>MSKVPSDIEIAQAAKMKPVMELARGLGIQEDEVELYGKYKAKISLDVYRRLKDKPDGKLILVTAITPTPAGEGKTTTSVGLTDALARLGKRVMVCLREPSLGPSFGIKGGAAGGGYAQVVPMEDINLHFTGDIHAVTYAHNLLAAMVDNHLQQGNVLNIDPRTITWRRVIDLNDRALRNIVIGLGGKANGVPRETGFDISVASEVMACLCLASDLMDLKERFSRIVVGYTYDGKPVTAGDLEAQGSMALLMKDAIKPNLVQTLENTPAFIHGGPFANIAHGCNSIIATKTALKLADYVVTEAGFGADLGAEKFYDVKCRYAGFKPDATVIVATVRALKMHGGVPKSDLATENLEALREGFANLEKHIENIGKFGVPAVVAINAFPTDTEAELNLLYELCAKAGAEVALSEVWAKGGEGGLELARKVLQTLESRPSNFHVLYNLDLSIKDKIAKIATEIYGADGVNYTAEADKAIQRYESLGYGNLPVVMAKTQYSFSDDMTKLGRPRNFTITVREVRL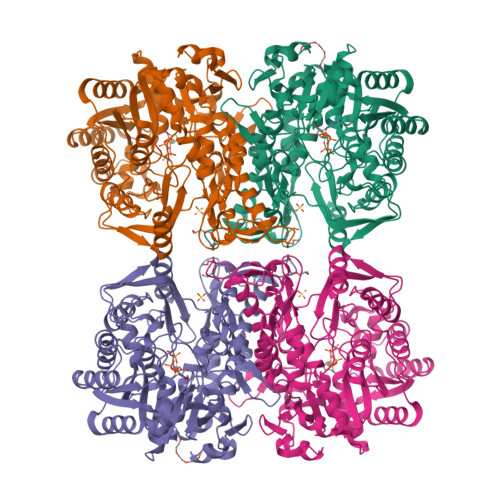SAGAGFIVPITGAIMTMPGLPKRPAACNIDIDADGVITGLF[2x]>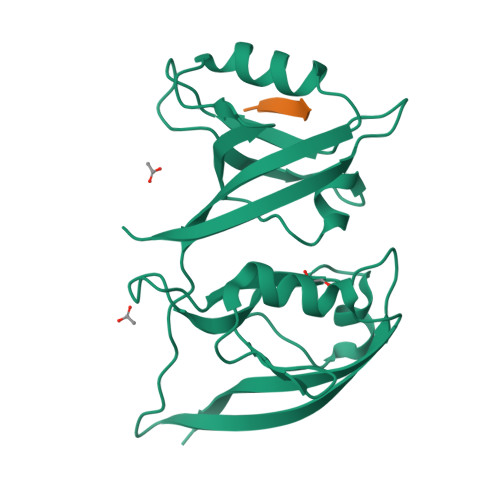GPGSFKGSTVVELMKKEGTTLGLTVSGGIDKDGKPRVSNLRQGGIAARSDQLDVGDYIKAVNGINLAKFRHDEIISLLKNVGERVVLEVEYELPPVSIQGSSVMFRTVEVTLHKEGNTFGFVIRGGAHDDRNKSRPVVITCVRPGGPADREGTIKPGDRLLSVDGIRLLGTTHAEAMSILKQCGQEATLLIEYDVSVMDS[2x];>[2x]NNLQDGTEV>GSSCQPGTTY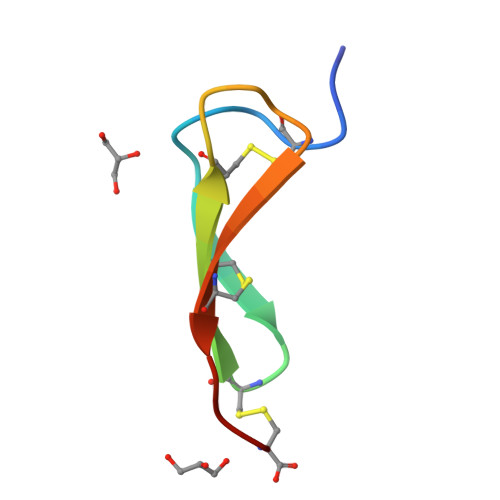QRGCNTCRCLEDGQTEACTLRLC[4x]> GSTKVYSQNGLVLHDDANFLEHELSYIDVLLDKNADQATKDNLRSYFA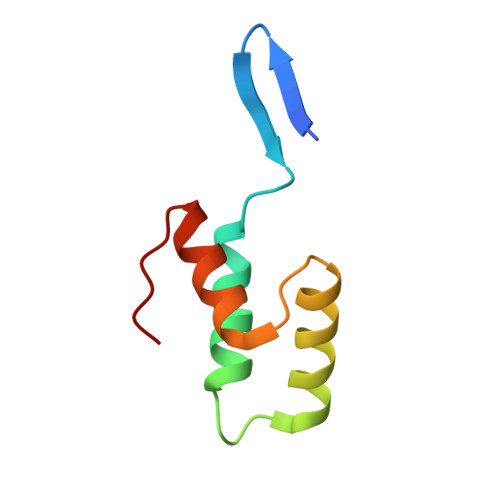DKGLHSIKDIINKAKQDGFDVSK>[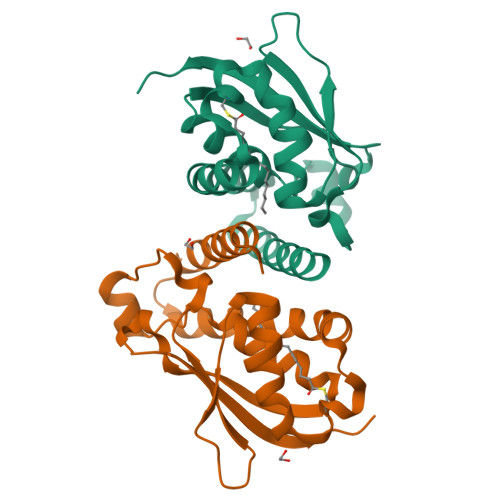6x]MAHHHHHHMSKLAKIGETTFNKIEKINSELLAMTYGSLVTQMLKDYEDVAAINTQLEKMGYKMGMRLIDEFMSKSGLSSGACREFKDTAESIAKVAFKMFLGINANVTNWSKDQTEYSIVFDENPLNDFVELPEPIKQKRLYYSNIICGVIRGALEMVLMRVECEYKKCPLLGDDQSEIRVRLKEYLRETVPSED> MNNNKAEADTSSSMADPETRPTYTTHHLAIPSGVT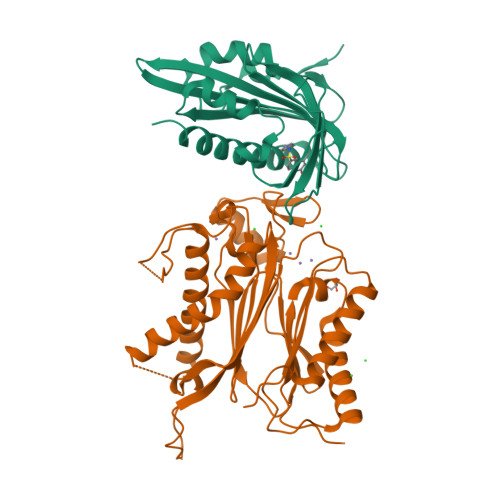QDEFDELKQSVVEFHTYQLSQNQCSSLLAQRIRAPNDVVWSIVRRFDQPQTYKHFIKSCSVSDNFTMAVGSTRDVNLISGLPAATSTERLDILDDDRQVLGISIIGGEHRLRNYRSVISVHGFNRDGAICTVALESYVVDVPEGNTEEDTRLFADTVVKLNLQKLVSVAESQVI;> RSVYELDCIPLWGTVSIQGNRSEMEDAFAVSPHFLKLPIKMLMGDHEGESPSLTHLTGHFFGVYDGHGGHKVADYCRDRLHFALAEEIERIKDELCKRNTGEGRQVQWDKVFTSCFLTVDGEIEGKIGRAVVGSSDKVLEAVASETVGSTAVVALVCSSHIVVSNCGDSRAVLFRGKEAMPLSVDHKPDREDEYARIENAGGKVIQWQGARVFGVLAMSRSIGDRYLKPYVIPEPEVTFMPRSREDECLILASDGLWDVMNNQEVCEIARRRILMWHKKNGAPPLAERGKGIDPACQAAADYLSMLALQKGSKDNISIIVIDLKAQRKFKTRT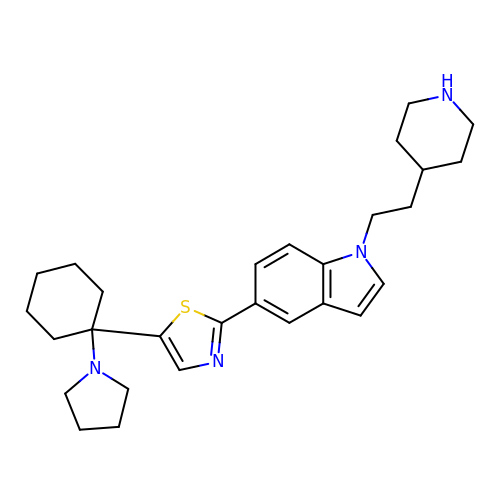1-[2-(piperidin-4-yl)ethyl]-5-{5-[1-(pyrrolidin-1-yl)cyclohexyl]-1,3-thiazol-2-yl}-1H-indole | C28 H38 N4 S | KBPMYBYNCAAYSC-UHFFFAOYSA-N> NSL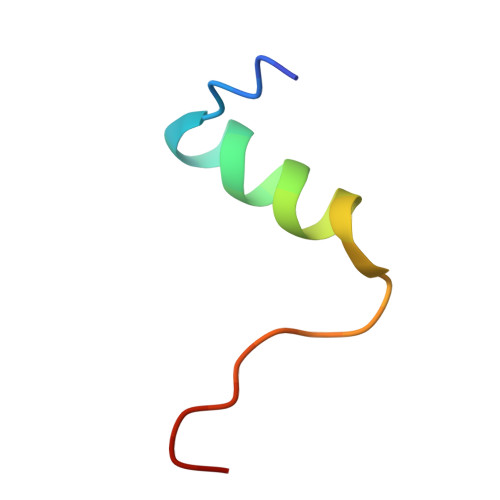RACGPALMDMLRVACPNGFNSMFAK> GPLGSMESYWDCKGIPILFRTVHAAVELAFTSQPGSISGYPSICRTTPLRTGPDERRQFPLTDTGAR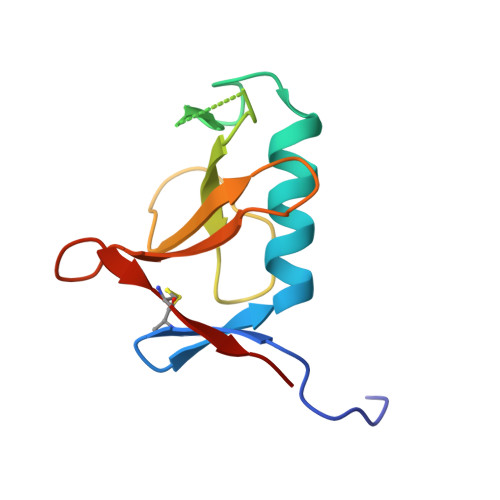WQGGGITYYVEATRDKRHCEVFGTAGGVYKCTLVLRD>SNAMMTKKERIAIQRSMAEEALGKLKAIRQLCGAEDSSDSSDMQEVEIWTNRIKELE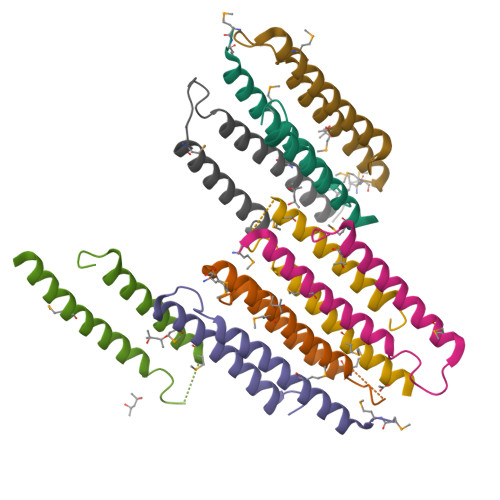DWLWGESPIA[8x]> NLFQFGEMILQKTGKEVVHSYAIYGCYCGWGGQGRAQDATDRCCFVHD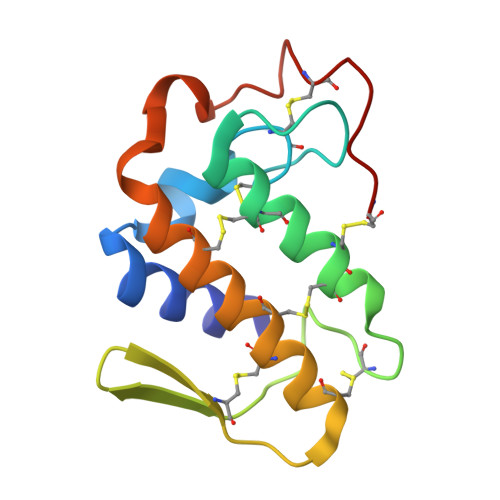CCYGTVNDCNPKTATYSYSFENGDIVCGDNDLCLRTVCECDRAAAICLGQNVNTYDKNYEYYSISHCTEESEQC> ETFSKIRVKP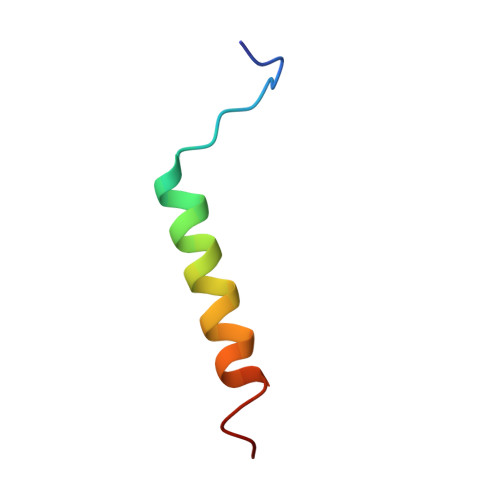EHVIGVTVAFVIIEAILTYGRF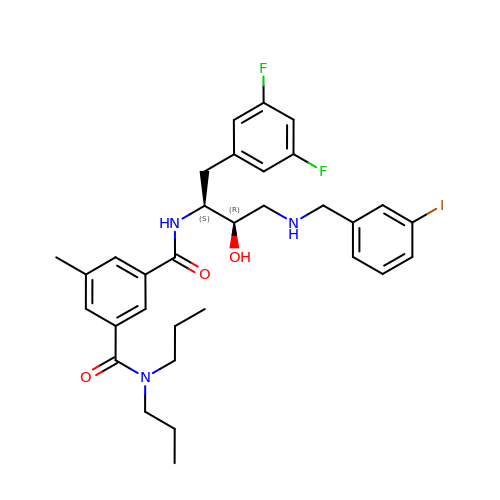N'-{(1S,2R)-1-(3,5-DIFLUOROBENZYL)-2-HYDROXY-3-[(3-IODOBENZYL)AMINO]PROPYL}-5-METHYL-N,N-DIPROPYLISOPHTHALAMIDE | C32 H38 F2 I N3 O3 | FSQSHDXWJKXBPP-XZWHSSHBSA-N>[3x]PCDSIVVAYYFCGEPIPYRTLVRGRAVTLGQFKELLTKKGSYRYYFKKVSDEFDCG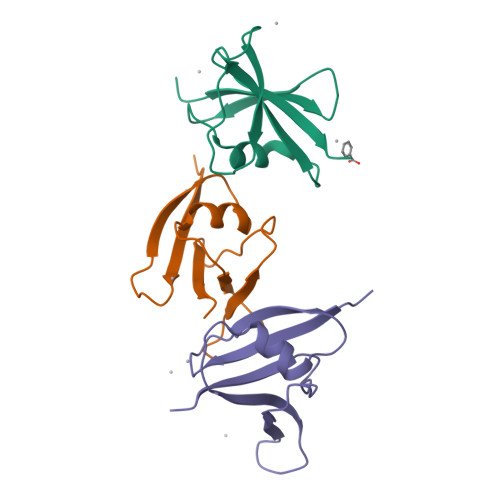VVFEEVREDEAILPVFEEKIIGKVEKVD>MARIRDVQGDITEFQGDAIVNAANNYLKLGAGVAGAILRKGGPSIQEECDRIGKIRVGEAAVTGAGNLPVRYVIHAAVLGDEPASLETVRK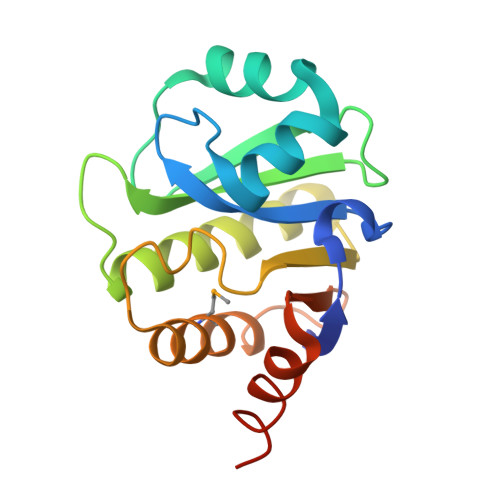ATKSALEKAVELGLKTVAFTVPGAWVGGLPAEAVRRVMVEEIKKAPDTLEVTGVHGTEKSAEACRRARLEHHHHHH[2x]> MAAIDKLVKASHLIDMNDIIREGNPTLRKVAEEVTFPLSEKEEILGEKMMQFLKHSQDPIMAEKLGLRGGVGLAAPQLDISKRIIAVLVPNVEDAQGNPPKEAYSLQEVMYNPKVVSHSVQDAALSDGEGCLSVDREVPGYVVRHARVTIEYFDKTGEKHRLKLKGYNSIVVQHEIDHIDGIMFYDRINEKNPFAVKEGLLILE;> MAR

PDFs are ubiquitous essential metalloenzymes which co-translationally remove the formyl group carried by the initiator methionine in bacteria, mitochondria and chloroplast. Here, we present and characterize a PDF enzyme issued from the bacterium Streptococcus agalactiae (SaPDF) which behaves as an excellent structural platform to describe PDF-inhibitor interactions. Like most other PDFs, SaPDF behaves as a monomer and its crystal structure reveals a classical PDF fold. In addition, SaPDF contains the typical insertions of type 2 PDFs12, including an eight-amino acids loop folded as an α-helix (insertion 2) and a long loop connecting strands β2 and β3 usually referred as the CD-loop (insertion 3).

The ligand binding site is localized at the interface between the N and the C sub-domains, as evidenced by the structures of the complexes between SaPDF and synthetic tripeptides. Crystal-soaking experiments were conducted with formylated peptides (Fo-Met-Ala-Ser and Fo-Met-Ala-Arg) but led to deformylated molecules in the crystal structures as previously reported for other PDFs2627. This is due to the ability of the enzyme to deformylate formylated substrates in the crystal packing. Peptides, which therefore represent deformylation reaction products, were found bonded to SaPDF through a high number of non-covalent interactions, which are similar to those found previously with Escherichia coli PDF (EcPDF). Indeed, the free N-terminal amine group coordinated catalytic ion and was hydrogen bonded to the catalytic residue Glu175. The hydrophobic methionine side chain fitted into a deep hydrophobic S1’ pocket composed of several conserved residues (Val71, Leu125, Glu129, Tyr167, Val171, His174). Finally, peptides were in a conformation mimicking a β-strand which was hydrogen-bonded with the main backbone peptide bond of Gly130 from conserved motif II (E129GCLS133), Val71 from conserved motif I (G70VGLAAPQ77), and Gly69 which preceds motif I, linking the two β-sheets from N- and C-terminal sub-domains.> MSDSDSDEGRVVEEPLPPHIIRFNDMAQHLLKKVIRQADVLIKENPQGLEKDIALNLVKFVKSQ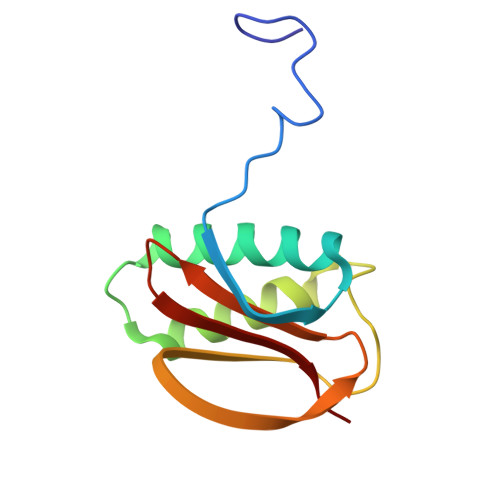PEFKIGDGEWQCIIGKNFGCSLTFDANVLAFFDLLPSRKSILLFKSG> NNTLWTGPKPEANCIIEYGKQNPDSKLTL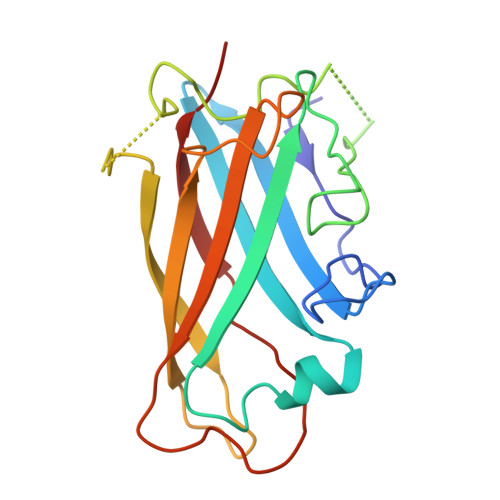ILVKNGGIVNGYVTLMGASDYVNTLFKNKNVSINVELYFDATGHILPDSSSLKTDLELKYKQTADFSARGFMPSTTAYPFVLPNAGTHNENYIFGQCYYKASDGALFPLEVTVMLNKRLPDSRTSYVMTFLWSLNAGLAPETTQATLITSPFTFSYIRED>[4x]MEF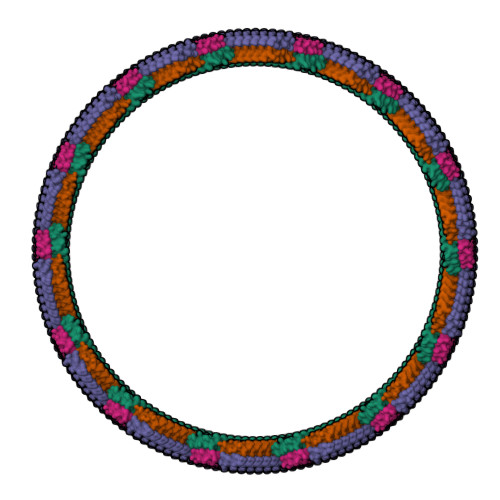VAKLFKFFKDLLGKFLGNN>MKISDGNWLIQPGLNLIHPLQVFEVEQQDNEMVVYAAPRDVRERTWQLDTPLFTLRFFSPQEGIVGVRIEHFQGALNNGPHYPLNILQDVKVTIENTERYAEFKSGNLSARVSKGEFWSLDFLRNGERITGSQVKNNGYVQDTNNQRNYMFERLDLGVGETVYGLGERFTALVRNGQTVETWNRDGGTSTEQAYKNIPFYMTNRGYGVLVNHPQCVSFEVGSEKVSKVQFSVESEYLEYFVIDGPTPKAVLDRYTRFTGRPALPPAWSFGLWLTTSFTTNYDEATVNSFIDGMAERNLPLHVFHFDCFWMKAFQWCDFEWDPLTFPDPEGMIRRLKAKGLKICVWINPYIGQKSPVFKELQEKGYLLKRPDGSLWQWDKWQPGLAIYDFTNPDACKWYADKLKGLVAMGVDCFKTDFGERIPTDVQWFDGSDPQKMHNHYAYIYNELVWNVLKDTVGEEEAVLFARSASVGAQKFPVHWGGDCYANYESMAESLRGGLSIGLSGFGFWSHDIGGFENTAPAHVYKRWCAFGLLSSHSRLHGSKSYRVPWAYDDESCDVVRFFTQLKCRMMPYLYREAARANARGTPMMRAMMMEFPDDPACDYLDRQYMLGDNVMVAPVFTEAGDVQFYLPEGRWTHLWHNDELDGSRWHKQQHGFLSLPVYVRDNTLLALGNNDQRPDYVWHEGTAFHLFNLQDGHEAVCEVPAADGSVIFTLKAARTGNTITVTGAGEAKNWTLCLRNVVKVNGLQDGSQAESEQGLVVKPQG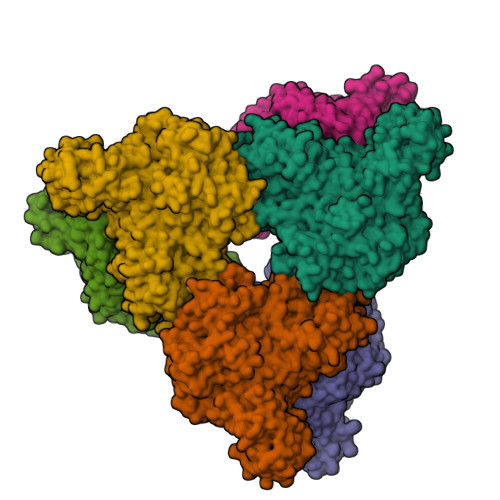NALTITLHHHHHH[6x]(2R)-2-{[6-(4-aminopiperidin-1-yl)-3,5-dicyano-4-ethylpyridin-2-yl]sulfanyl}-2-phenylacetamide 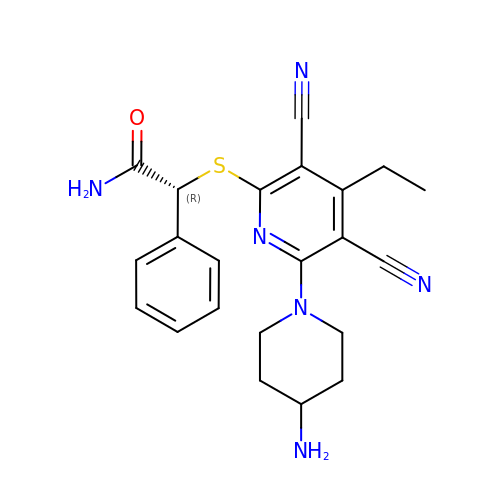| C22 H24 N6 O S | KNKHRZYILDZLRE-LJQANCHMSA-N> HAADRIARLPGQPAVDFDMYSGYITVDEGAGRSLFYLLQEAPEDAQPAPLVLWLNGGPGCSSVAYGASEELGAFRVKPRGAGLVLNEYRWNKVANVLFLDSPAGVGFSYTNTSSDIYTSGDNRTAHDSYAFLAKWFERFP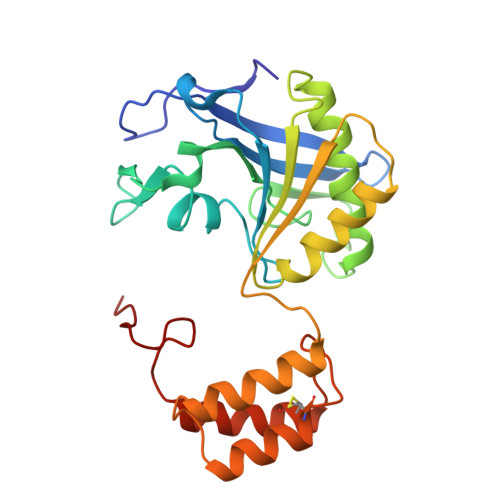HYKYRDFYIAGESYAGHYVPELSQLVHRSKNPVINLKGFMVGNGLIDDYHDYVGTFEFWWNHGIVSDDTYRRLKEACLHDSFIHPSPACDAATDVATAEQGNIDMYSLYTPVCNI> MGATLSAPKKKKTQVGASWVGNESENPFDLALNKKDRTLLRETWQRLDDPKDIVGLIFLDIVNDIEPDLKKVFGVDRAPRAAMLKMPKFGGHILRFYEFMEQLTSMLGTSENLTGAWQLVRKTGRSHVRQGFLEQNQNQMEKNYFEIVINVFIERLIPFLTGEQELPSSEGKENKKVRFAQNYTTSQITDVWKKFLNTVISQMTDSFELERAKQKSAQTTKALAPHQHIEISERKKKRVAEKQSEIENTAVSNEPKAQEQMFEDPF

In this study, we identified a novel role within the globin superfamily by showing that GLB-12 of C. elegans functions as a redox signalling protein in the reproductive system. We observed that GLB-12 shows a hexacoordinated haem, extremely low ligand affinity, a relatively low redox potential and the ability to transfer electrons to other molecules in a continuous manner. We found that, by using structural, biochemical and mutational approaches, GLB-12 actively converts O2 to O2.−, which in turn is used as a redox signalling molecule. Based on our findings, we propose a model whereby GLB-12 acts as a superoxide generator in the somatic gonad, after which this O2.− signal is modulated directly or indirectly by an intracellular and an extracellular SOD, creating a transmembrane H2O2 gradient that acts as a redox signal.

The crystal structure of the GLB-12 globin domain, refined to 1.65 Å resolution, further supported our current findings. It confirmed haem hexacoordination, with strong Fe-N bonds with the distal His92 and the proximal His127 residues. The proximal His127 is highly exposed to the solvent, which is the result of a hydrogen bond between the A-propionate of the haem to Ser126 OH. As a result, two water molecules are hosted at the entrance of the proximal site (hydrogen bonded to Ser126 OG and to Gln130 NE2, respectively), and four additional water molecules and one acetate ion fall next to the propionate. This exposure to a polar aqueous environment would favour oxidation of the ferrous haem, which is consistent with the low GLB-12 redox potential reported. In addition, residues Phe89 and Phe96 (surrounding the distal His92) are part of a wide cluster of aromatic/hydrophobic residues (Val54, Phe58, Leu59, Val62, Phe73, Phe152) (not highlighted). These could restrict E-helix movements required to achieve a pentacoordinated haem and would thereby limit ligand binding. Additionally, this aromatic/hydrophobic residue cluster creates a tunnel of about 50 Å3 in the globin domain, nestled among the B-, E-, and G-helices. Interestingly, this otherwise apolar tunnel shows a strong negative charge distribution at the solvent exit (resulting from residues Asp48, Asp49, Asp52 and Glu165). Further, while the haem pocket in globins usually prevents haem iron oxidation by creating a hydrophobic environment, in GLB-12 three polar amino acids (Lys88, Arg95 and Arg129) are located at the edge of the haem cavity, possibly to enhance solvent access to the haem and stimulate haem iron oxidation and O2.− production.> PISPIETVPVKLKPGMDGPKVKQWPLTEEKIKALVEICTEME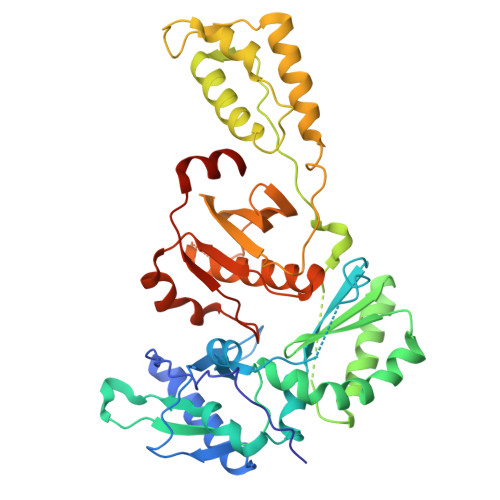KEGKISKIGPENPYNTPVFAIKKKDSTKWRKLVDFRELNKRTQDFWEVQLGIPHPAGLKKKKSVTILDVGDAYFSVPLDEDFRKYTAFTIPSINNETPGIRYQYNVLPQGWKGSPAIFQSSMTKILEPFRKQNPDIVIYQYMDDLYVGSDLEIGQHRTKIEELRQHLLRWGLTTPDKKHQKEPPFLWMGYELHPDKWTVQPIVLPEKDSWTVNDIQKLVGKLNWASQIYPGIKVRQLCKLLRGTKALTEVIPLTEEAELELAENREILKEPVHGVYYDPSKDLIAEIQKQGQGQWTYQIYQEPFKNLKTGKYARMRGAHTNDVKQLTEAVQKITTESIVIWGKTPKFKLPIQKETWETWWTEYWQATWIPEWEFVNTPPLVKLWYQLEKEPIVGAETF> MMRKSVTFLRRGKPRPRAGMFPDKYRRVPMLLKPQQGGQQYFNHFLIRSTNDRLTQQDVDNASGQAHSFISPQLPQMDWRNMSARSSEESIREEMRQLAENDVMQHQRVFNERMWYEKEEEHRMKARSCPEETSEHAXSNDGAVPPPRVLGG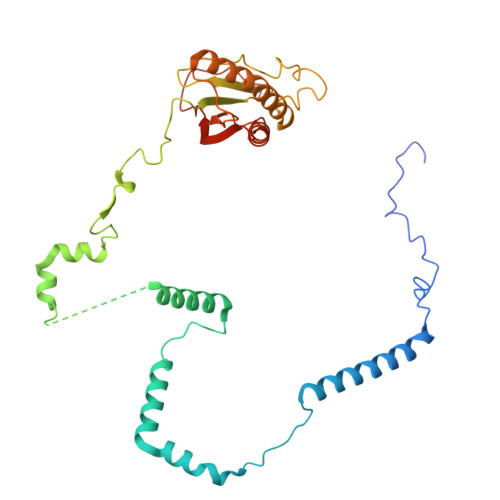DYFKTRFGYSLVKNSEMTQGPVDYSQLDMWGEMPRYTSDMVFLYLVSRRRNTYAVAYTYEGKRILNTYTAGNRGLKGGDRGFRSEGSTDNGHQVTSMYLNDLLPKLREMRASEGRPMGRGEKVELVVRVMGFYNGRQGAVRAVQDRANEFHVRYFEDITPFPLNGPKMPRGVFK>[2x]MGSSHHHHHHSQDPNSSSARLQVDKLAMSPVSVAQRNTGIWAVVPLKAPECAKTRLAGVLSHAARQALFFSMASHVIGTLRASPRIASLLVVTPSESTAEMARAAGAEILWGPPDEGMANACSRAMAHIAAAGGERVMFVPGDLPLLDEAAIDMLSRAPVDAIGMAPNRDGHGTNGLICRPGAIPLFFSGPSFSAHQNAARRAGIDVWVVRSREWALDVDLPADLEEFESSVRDAKRRVLCQN

Coenzyme F420 is a microbial redox cofactor that mediates diverse physiological functions and is increasingly used for biocatalytic applications. 3PG-F420 is formed via activation of 3-phospho-d-glycerate (3-PG) by CofC, but the structural basis of substrate binding, its evolution, as well as the role of CofD in substrate selection remained elusive. Instead, enzyme assays revealed that 3-phospho-d-glycerate (3-PG) is activated by CofC, presumably forming the short-lived intermediate 3-(guanosine-5′-diphospho)-d-glycerate (GPPG), which is further transferred to the FO core by the action of CofD. Here, we present a crystal structure of the 3-PG-activating CofC from Mycetohabitans sp. B3 and define amino acids governing substrate specificity.

From diffraction data collected to 2.4 Å the crystal structure could be solved by molecular replacement with a model of two superimposed structures (Mtb- FbiD and Methanosarcina mazei CofC, Mmaz-CofC). The overall structure was similar to the known homologs with the core of the single-domain protein being a six-stranded mixed β-sheet. Intriguingly, after initial refinement both molecules in the asymmetric unit independently showed unambiguous difference density for GPPG, the reaction product of GTP with 3-PG, completely immersed into the active site pocket. Each building block of GPPG (i.e., guanine, ribose, phosphate, and glycerate) is bound by several interactions. Guanine is distinguished from adenine by two H-bond donors to its oxygen (main-chain nitrogen of V65 and P86) and two H-bond acceptors to its amino group (main-chain carbonyl group of E89 and G90). The α- and β-phosphates are bound by two Mg2+ ions, which in turn are positioned by three aspartates (D116, D193, D191) similarly as had been shown for FbiD before. Hence, GPPG is tightly bound, in fact, it turned out to be still quantitatively bound after purification of the protein from E. coli cell lysate, where both substrates were present. The 3-PG moiety is primarily bound by H-bonds with the side chain of S165 to the carboxy group, apparently a highly conserved binding site of the carboxylate of the C3-acid as known from Mtb-FbiD. More interactions with the carboxy group arise from H-bonds with main-chain nitrogen atoms of T147 and S162, the latter being critical for selective 3-PG activation. The reason why the 3-PG adopts a new orientation is the main-chain rotation of S162, the CA and CB of which then squeeze the 3-PG into the productive conformation.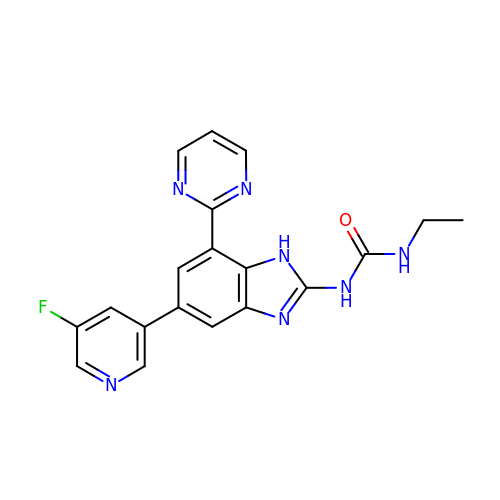1-ethyl-3-[5-(5-fluoropyridin-3-yl)-7-(pyrimidin-2-yl)-1H-benzimidazol-2-yl]urea | C19 H16 F N7 O | FKCGKEHVIVGGDU-UHFFFAOYSA-N Androsterone | 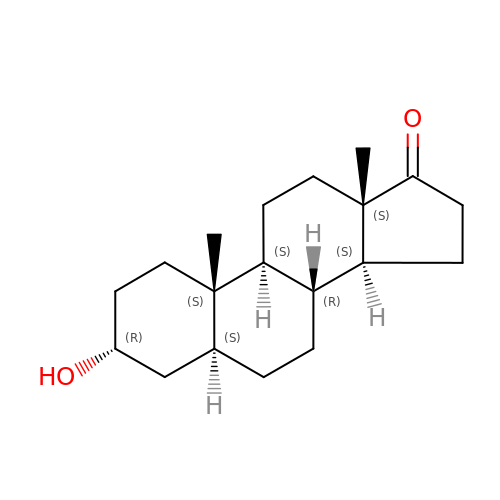C19 H30 O2 | QGXBDMJGAMFCBF-HLUDHZFRSA-N>QLRYSVVEESEPGTLVGNVAQDLGLKGTDLLSRRLRLGSEENGRYFSLSLVSGALAVSQKIDRESLCGASTSCLLPVQVVTEHPLELTRVEVEILDLNDNSPSFATPDREMRISESAAPGARFPLDSAQDPDVGTNTVSFYTLSPNSHFSLHVKTLKDGKLFPELVLEQQLDRETQARHQLVLTAVDGGTPARSGTSLISVIVLDVNDNAPTFQSSVLRVGLPENTPPGTLLLRLNATDPDEGTNGQLDYSFGDHTSETVKNLFGLDPSSGAIHVLGPVDFEESNFYEIHARARDQGQPAMEGHCVIQVDVGDAN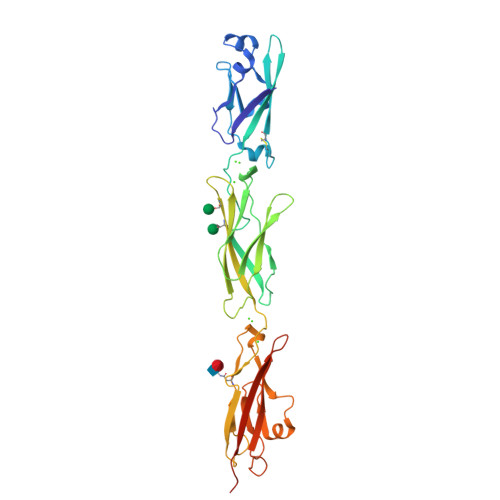DHHHHHHHH[3x]>MACPLEKALDVMVSTFHKYSGKEGDKFKLNKSELKELLTRELPSFLGKRTDEAAFQKLMSNLDSNRDNEVDFQEYCVFLSCIAMMCNEFF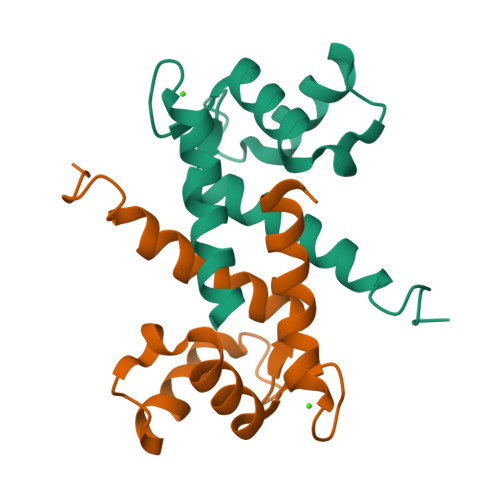EGFPDKQPRKK[2x]Fixed targets (‘chips’) offer efficient, high-throughput microcrystal delivery for serial crystallography at synchrotrons and X-ray free-electron lasers (XFELs). Within this family, sheet-on-sheet (SOS) chips offer noteworthy advantages in cost, adaptability, universality and ease of crystal loading. We describe our latest generation of SOS devices, which are now in active use at both synchrotrons and XFELs. In essence, SOS dispenses with a patterned solid support pane and simply sandwiches a thin layer of crystal slurry (typically 20 µm thick) directly between two transparent polymer films (each typically 2–6 µm thick) to fill the entire window of the chip.

In many instances, a significantly higher yield of indexed lattices per chip is desired. The sample layer is sealed between the two SOS films by clamping them together against an M42x1 O-ring. The large SOS chip has also been used at the ID29 SMX endstation, both to collect data for model systems and with bona fide samples. Excellent high-resolution data can be obtained (the statistics of a thaumatin dataset are given in Tables S4 and S5 of the supporting information). We typically use 2.5–3 µm-thick Etnom sheets for crystals in aqueous solutions and 6 µm-thick Mylar sheets for crystals in LCP. To prevent sample settling yet allow leeway in adjusting the crystal slurry layer thickness, we often add 1.5–2% hy­droxy­ethyl cellulose to the mother liquor. Our layers of crystalline slurries are typically 20–30 µm thick. SOS chips are unique in their cost effectiveness and in their ease and versatility of use with crystals of both soluble and membrane proteins, as grown in both low-viscosity (aqueous solutions) and high-viscosity media (LCP).

> ATFEIVNRCSYTVWAAASKGDAALDAGGRQLNSGESWTINVEPGTKGGKIWARTDCYFDDSGSGICKTGDCGGLLRCKRFGRPPTTLAEFSLNQYGKDYIDISNIKGFNVPMDFSPTTRGCRGVRCAADIVGQCPAKLKAPGGGCNDACTVFQTSEYCCTTGKCGPTEYSRFFKRLCPDAFSYVLDKPTTVTCPGSSNYRVTFCPTA> GCG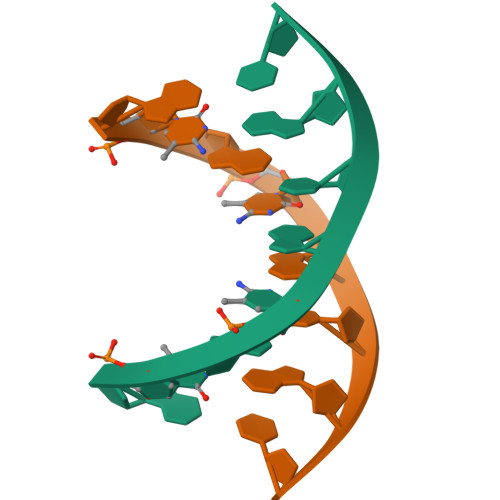CGCGC> SRRFERDPTIPPDSIKVYSRTLFLGGIT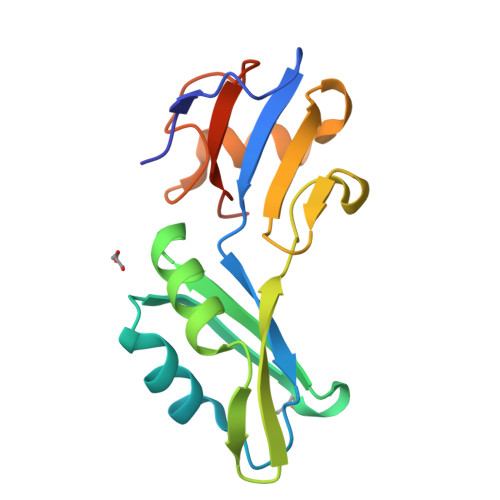RSVREPVLRSMFERFGSVQSLILNHNYRHGFLKMFRRDAAEKAQVAMENVPFADTTIRTKWSVGFGPRECSDFSTGISVIPIRLLTDADRTWLVTAEYGGTGGLPITPGIALDEPDIEIGLGISS TERT-BUTYL 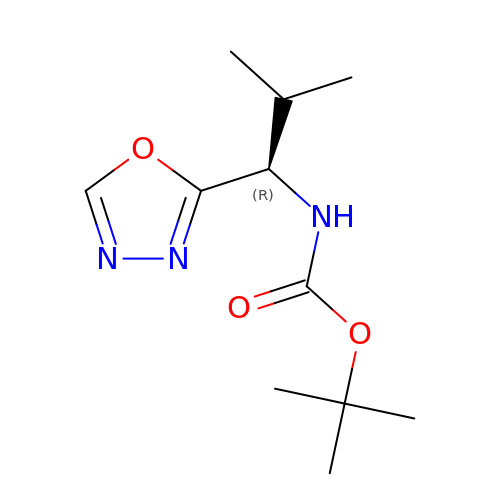[(1R)-2-METHYL-1-(1,3,4-OXADIAZOL-2-YL)PROPYL]CARBAMATE | C11 H19 N3 O3 | PARUDDGQWSBIIO-MRVPVSSYSA-N2-[3-(methoxymethyl)phenyl]-N-[4-(1H-pyrazol-4-yl)phenyl]acetamide 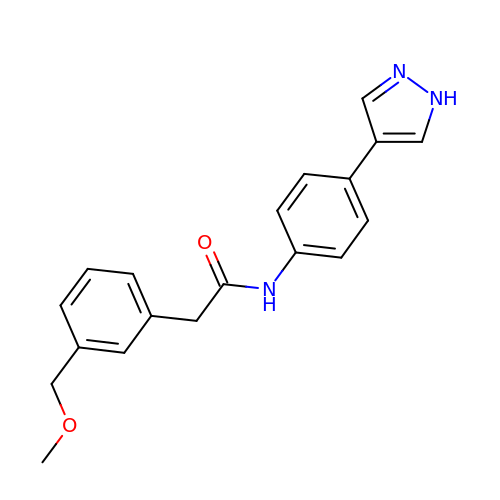| C19 H19 N3 O2 | LTOKSVFUTQZXGU-UHFFFAOYSA-N>PSDEAMTVRPVDQRPSLDSTFERLSKLQPTATSCLAKDSESLFNDLCSVFLSAAVSESDLERFDATPVLSRPKAPSNSFYLSFYLRVWCGPYPTLAKVAALERVKTRLKEGDCVDKDFQAIFPYCIAALSDPAKKVRRAAADLVAVLGSAYKSLEKSQQLWAAKDLYGKTGTTSPLDKDALKALIRSVLIPCLEESVLHEDHVVAALVGALESSKDSENKNADKRHLSHSARLSIFKFLCGHVVETPLLAVKLRLLRSLNQIRRISGTTRTDLLLPLLRWWAGLSANEAAELAAQESVDVPAIDDAVVDVVVPNHAAGLEAFFQLVKEAIRPGLLQAIFARIAKMWPSMKSDTKYSTAKTLFELTQDPKLNAEQSDVITEAVEVLRKVDLTTDILHYFIDS[2x]

The 5' region of pre-rRNA that consists of the 5' external transcribed spacer (5' ETS), 18S rRNA and the internal transcribed spacer 1 (ITS1) is co-transcriptionally packed into a terminal ball of ~40 nm in size. These particles represent the earliest assembly intermediates of 40S and are known as the 90S pre-ribosome or the SSU processome. Within 90S, the pre-rRNA is cleaved at sites A0 and A1 in the 5' ETS and site A2 in the ITS1, yielding a 20S pre-rRNA intermediate. The fully assembled 90S contains an unprocessed pre-18S rRNA, U3 snoRNA, approximately 51 assembly factors and 18 r-proteins with a molecular mass of 5.0 megadaltons.

The EM densities were docked with the available crystal structures of yeast 40S ribosome and AFs or homology models of AFs. Utp10 is a large protein (1769 residues) with mostly α-helices by prediction. In the EM map, the M domain is continued by an elongated density that should correspond to the C-terminal region (C domain) of Utp10. In addition, the UTPA protein Utp10 adopts an extended superhelical structure pointing upwards, forming the large arch. The WD domain of Utp5 contacts the WD domain of Utp4 and the M domain of Utp10. The exposed H1 lies over the tandem WD domains of Utp17 and contacts the CTD of Utp9 by its base and the M domain of Utp10 by its tip.>[4x]MVLMIVSGRSGSGKSVALRALEDMGFYCVDNLPVVLLPDLARTLADREISAAVSIDVRNMPESPEIFEQAMSNLPDAFSPQLLFLDADRNTLIRRYSDTRRLHPLSSKNLSLESAIDKESDLLEPLRSRADLIVDTSEMSVHELAEMLRTRLLGKRERELTMVFESFGFKHGIPIDADYVFDVRFLPNPHWDPKLRPMTGLDKPVAAFLDRHTEVHNFIYQTRSYLELWLPMLETNNRSYLTVAIGCTGGKHRSVYIAEQLADYFRSRGKNVQSRHRTLEKRKP

GlmZ stimulates translation of the mRNA encoding GlcN6P synthtase in Escherichia coli, but when bound by RapZ protein, the sRNA becomes inactivated through cleavage by the endoribonuclease RNase E. Here, we report the cryoEM structure of the RapZ:GlmZ complex, revealing a complementary match of the RapZ tetrameric quaternary structure to structural repeats in the sRNA. RapZ then presents GlmZ to the endoribonuclease RNase E in a manner that directs cleavage within the base‐pairing site of the sRNA, thereby inactivating it and silencing synthesis of the synthase (Göpel et al, 2013; Gonzalez et al, 2017; Durica‐Mitic et al, 2020). The protomers have two domains of roughly equal size: the N‐terminal domain (NTD) bears Walker A and B motifs and resembles an adenylate kinase, while the C‐terminal domain (CTD) bears structural similarity with the sugar‐binding domain of phosphofructokinase. Here, we have elucidated the structures of both the binary complex of RapZ:GlmZ and the ternary complex of the RNase E catalytic domain (RNase E‐NTD), RapZ and GlmZ, using electron cryo microscopy (cryoEM).

A map of the binary complex was obtained at 4.4 Å resolution based on Fourier shell correlation (Fig EV3; Table EV1). This map provides an envelope that accommodates well a crystal structure of the RapZ tetramer and confirms the distinctive quaternary structure observed earlier (Gonzalez et al, 2017). Remaining density allowed for the building of the first two stem loops of GlmZ RNA (SLI and SLII). The RNA stem loops are primarily contacted by the CTD dimers of RapZ; SLI interacts with the CTD dimer formed by chains C and D, whilst SLII interacts with the dimer formed by chains A and B. For both stem loops, the path of the RNA across the CTD dimer has approximately two‐fold symmetry, and the conformation of the duplex changes from A‐form to a highly underwound helix near the dyad symmetry axis (roughly between residue K170 of chains A and B, respectively). Several basic residues (K170, R184, K194, R196, R211, R238, K251) form patterns of positive charges on the CTD surface providing a favourable electrostatic match to the path of the sRNA. The phosphate backbones of each of the two stem loops of GlmZ align with corresponding putative ligand‐binding pockets formed by the CTDs of chains A/B and C/D, respectively. The Walker A and B motifs located in the N‐terminal domain of RapZ are not positioned to contact the RNA substrate, instead they appear to run along the opposite diagonal of the RapZ tetramer to the RNA. The RNase E cleavage site in GlmZ, which resides within the single‐stranded region located between SLII and SLIII, is not resolved in our cryoEM maps and is likely disordered. The binary complex is also likely to resemble the postcleavage product, where only the SLI and SLII are bound by RapZ.>CGCGAATT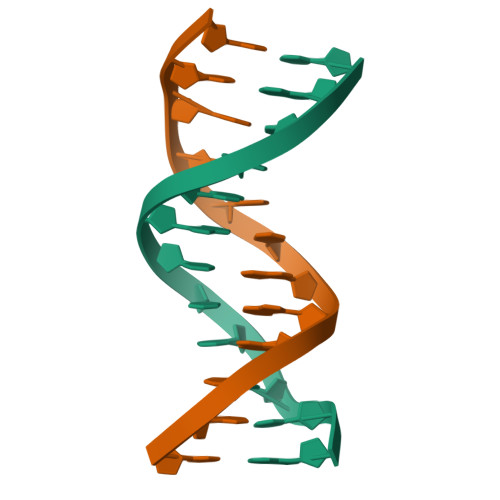TGCG[2x]> PA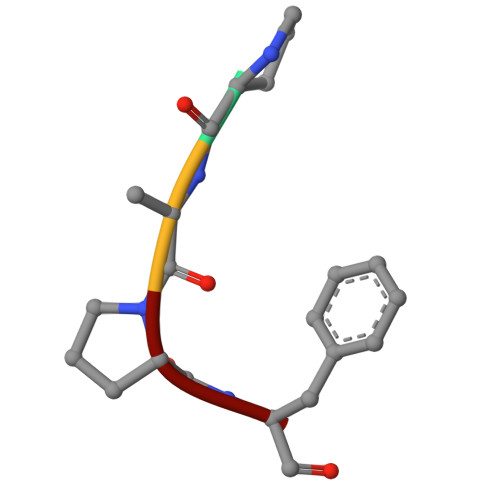PF> MGHHHHHHLYFQGMNRPSFNEAWLAFRKVNHSVADVGSIIGGNVGKNITGGYFQNACPIRMSYVLNATGFPIARNSPYAKVSGADNKFYIYRVNDMIDYLTHTMGKPDLIVNNPKQSDFIGKKGIIVVKGHGWSNARGHVTLWNGSICSDQCHLLNDPDNGPFVPEVGTLWILP;> QEALTTQYSQSELLKNWALSHCLALVYKDDVVKNDARATASAYLEYGKQSVEIYHEIDEIAKKYSGLKYNGSISSDFNTMKC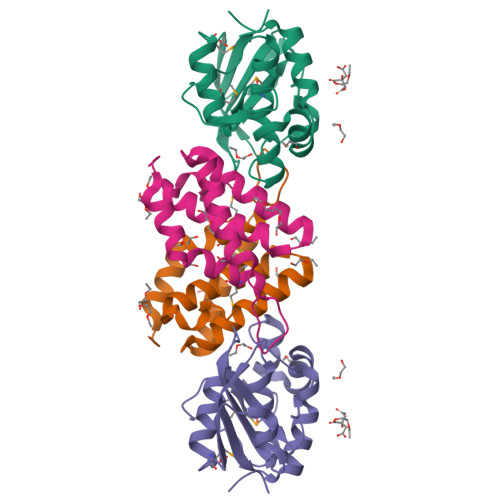IDFIHDRELNELIKRRVEK BrlR, a member of the MerR family of multidrug efflux pump activators, consists of a structurally conserved N-terminal DNA-binding domain and a C-terminal GyrI-like binding domain. BrlR mediates the antibiotic resistance of P. aeruginosa by activating the expression of multidrug efflux pumps and repressing PhoPQ activation. The monomer can be divided into three domains: the N-terminal DNA-binding domain (residues 1–75), which adopts a winged helix-turn-helix fold; the long central α-helical linker (residues 76–119), which connects two terminal domains; and the C-terminal multidrug-binding domain (residues 120–270). Our most striking finding is that BrlR is not only a pyocyanin receptor but it is also a dual receptor that is responsive to both c-di-GMP and pyocyanin.

Subsequently, the structure of apo-BrlR is determined by molecular replacement (MR) using a protein monomer of BrlR–c-di-GMP complex as the search model. The final model of apo-BrlR is refined to 3.1 Å resolution and contains four BrlR molecules in the asymmetric unit. Two full-length monomers (A and D) can be traced, and the other two (B and C) have the same interruptions (residues 32–36 and residues 138–143). Four BrlR subunits assemble into a stable homotetramer which is composed of two cross-stacked dimers (AD, BC). Unlike other MerR-like proteins, BrlR forms a distinctive dimer of dimers. The head-to-tail interaction of BrlR in a tetramer occurs only between two adjacent dimers (AC vs. BD). Helix α1 and the subsequent turn of the HTH motif occupy the groove of another BrlR-C domain in the BrlR tetramer, with helix α3 interacting with helix α7′ of the BrlR-C domain. The unusual interface of BrlR tetramer causes most of its DNA-binding region blocked by the multidrug-binding domains from their tetrameric partners, thus indicating a lower DNA-binding ability. To our knowledge, the tetrameric BrlR reported here provides the first example of a self-blocked MerR-like transcriptional regulator. The blocked HTH motif and the long distance between two recognition helices hinder BrlR to approach and bind DNA, thus resulting in a very low DNA-binding capability of BrlR.

>[4x]GSMLTIGQLARIFEISTKTLRHYDAIGLFVPARTGSDNGYRYYQPEQIEQLSRILALRRLDVPLEAIDRLKRDGALDDPQRLRHFLQRHQHTLREEISARQRLLAELDRTLATLAHWRIRNMHARIVERPAFSVVGMEYFGSAPGDTIGQLWERFIPREHEIAGKHDPEVSYGICAQQPNGEFHYVAGFEVQEGWPVPEGMVRFQVPAQKYAVFTHKGTAPQIAESFQAIYSHLLAERGLEPKAGVDFEYYDQRFRGPLDPNSQVDLYIPIY(2R)-2,3-dihydroxypropyl dodecanoate | C15 H30 O4 | 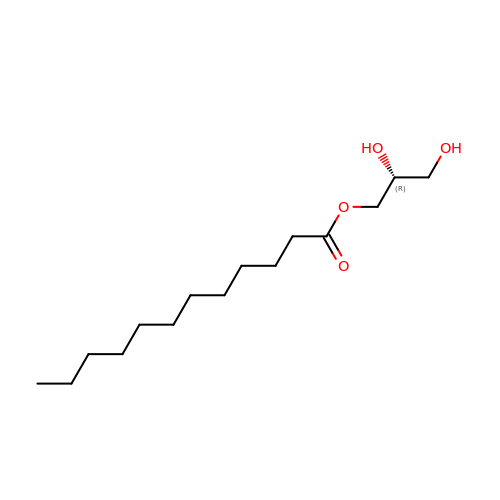ARIWANIATODDMH-CQSZACIVSA-N> DVSFRLS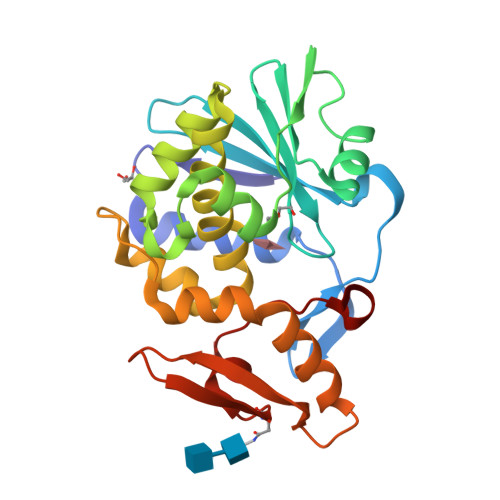GADPSSYGMFIKDLRNALPHTEKVYNIPLLLPSVSGAGRYLLMHLFNYDGNTITVAVDVTNVYIMGYLALTTSYFFNEPAADLASQYVFRSARRKITLPYSGNYERLQIAAGKPREKIPIGLPALDTAISTLLHYDSTAAAGALLVLIQTTAEAARFKYIEQQIQERAYRDEVPSSATISLENSWSGLSKQIQLAQGNNGVFRTPTVLVDSGGNRVQITNVTSNVVTSNIQLLLNTKNI N-[4-(4-methylpiperazin-1-yl)phenyl]acetamide | C13 H19 N3 O | 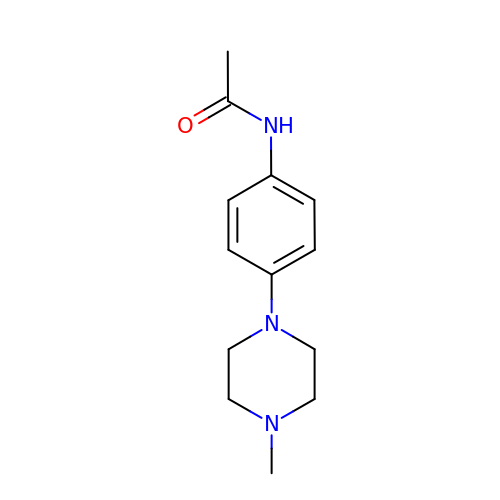QAEVFGOUSCYAPU-UHFFFAOYSA-N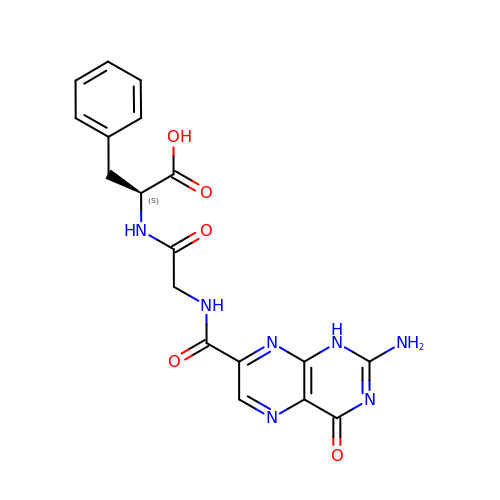N-[(2-amino-4-oxo-1,4-dihydropteridin-7-yl)carbonyl]glycyl-L-phenylalanine | C18 H17 N7 O5 | XYQCEJDIFQQSAN-JTQLQIEISA-N~{N}4-[(4-chlorophenyl)methyl]-~{N}4-cyclopentyl-~{N}1-(phenylmethyl)-~{N}1-(piperidin-4-ylmethyl)benzene-1,4-disulfonamide | C31 H38 Cl N3 O4 S2 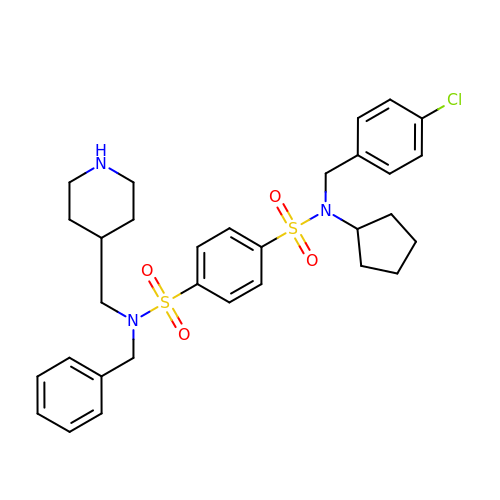| SCLQBRLPJHXGKJ-UHFFFAOYSA-N> 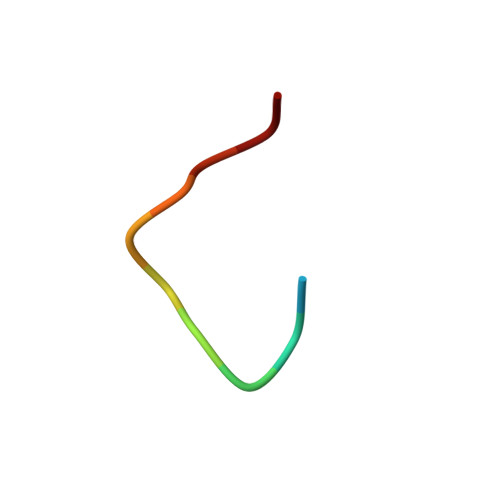XFVYSAVCLYV D-PHENYLGLYCINE | C8 H9 N O2 | 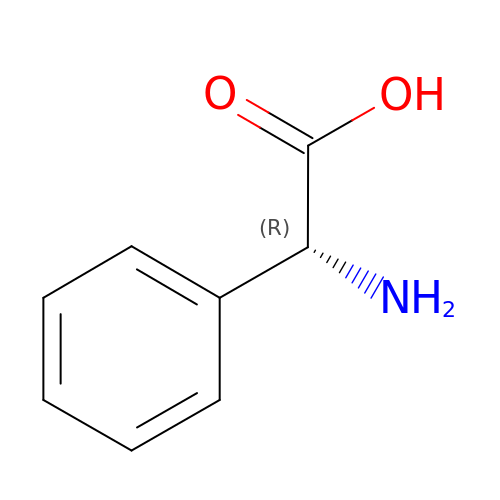ZGUNAGUHMKGQNY-SSDOTTSWSA-N>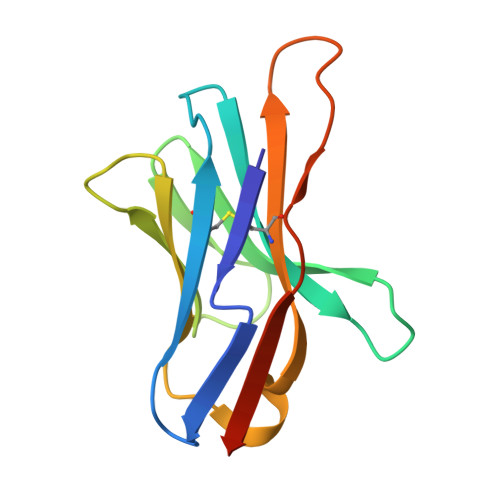 SLTFYPAWLTVSEGANATFTCSLSNWSEDLMLNWNRLSPSNQTEKQAAFSNGLSQPVQDARFQIIQLPNRHDFHMNILDTRRNDSGIYLCGAISRHPKAKIEESPGAELVVTERILE>[2x]LPEQIDWRKKGAVTPVKNQGKCGSCWAFSTVSTVESINQIRTGNLISLSEQQLVDCNKKNHGCKGGAFVYAYQYIIDNGGIDTEANYPYKA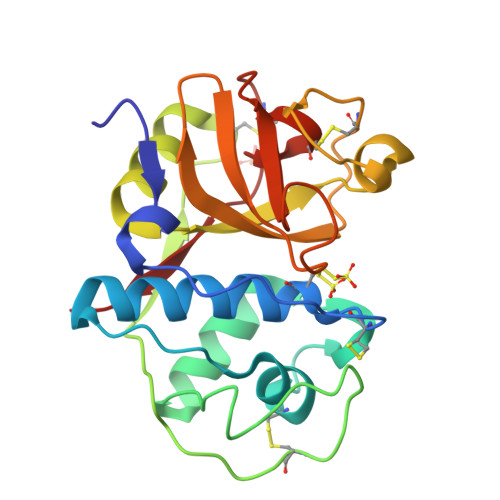VQGPCRAAKKVVRIDGYKGVPHCNENALKKAVASQPSVVAIDASSKQFQHYKSGIFSGPCGTKLNHGVVIVGYWKDYWIVRNSWGRYWGEQGYIRMKRVGGCGLCGIARLPYYPTKA Nuclear abundant poly(A) RNA-binding protein (Nab2) is an essential multidomain hnRNP that is required for the nuclear export of poly(A) mRNA in S. cerevisiae. The Nab2 protein has a modular structure based on four functional domains:23 a unique N-terminal domain of approximately 100 residues, a glutamine-rich linker, an RGG domain, and a Zn-finger domain. Our studies demonstrate that the N-terminal domain of Nab2 is both necessary and sufficient to mediate interaction with Mlp1. The Nab2 N-terminal domain has a fold based on a five-helix bundle that is analogous to the PWI fold found in SRm160 and other nucleic acid binding proteins, although it does not retain the nucleic acid binding function seen in other PWI domains.

We also obtained P43212 symmetry crystals of the Nab2 N-terminal domain that diffracted past 1.8 Å resolution in-house. We used the solution NMR structure of this domain as a model for molecular replacement and, after trying a number of different models containing different fragments of the structure, were able to obtain a unique solution using residues 7–82 (corresponding to helices H1–H4). After solvent flattening, the electron density enabled residues 6–94 to be built to produce a structural model that had an R-factor of 20.7% (Rfree = 26.4%) and excellent geometry after iterative cycles of refinement and rebuilding. The crystal and solution structures of the N-terminal domain of Nab2 were very similar for helices H1–H4 and superimposed with a Cα rmsd of 1.2 Å. However, the position of helix H5 varied significantly between the two structures as a result of a rigid-body rotation of the order of 25°. This difference in the position of helix H5 could have been the result of crystal packing or might have been a consequence of partial proteolysis as it was only possible to trace the chain in the crystal structure as far as residue 94, whereas in the solution structure, this helix extended to residue 99. Inspection of the solution and crystal structures of the Nab2 N-terminal domain showed the presence of a hydrophobic patch centered on Phe72 and Phe73, suggesting that this region of the surface might represent a putative protein:protein interaction interface. Phe73 in particular was completely exposed on the surface of the protein. Overall, the mutagenesis results are consistent with Phe73 forming a crucial component of the interaction interface between Nab2 and Mlp1 and hydrophobic interactions making an important contribution to the interface.

> MSQEQYTENLKVIVAEKLAGIPNFNEDIKYVAEYIVLLIVNGGTVESVVDELASLFDSVSRDTLANVVQTAFFALEALQQGESAENIVSKIRMMNAQSLGQSDI> TRIKITELNPHL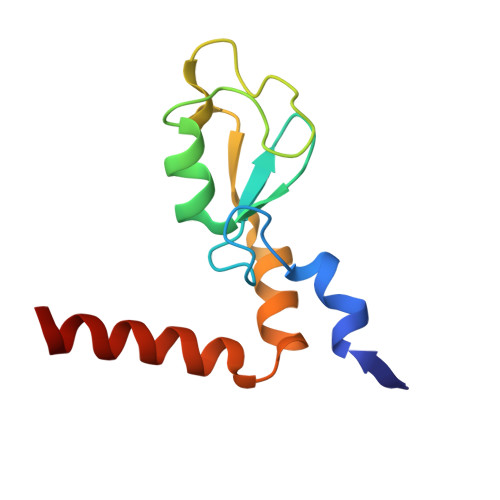MCVLCGGYFIDATTIIECLHSFCKTCIVRYLETSKYCPICDVQVHKTRPLLNIRSDKTLQDIVYKLVPGLFKNEMKRRRDFYAAH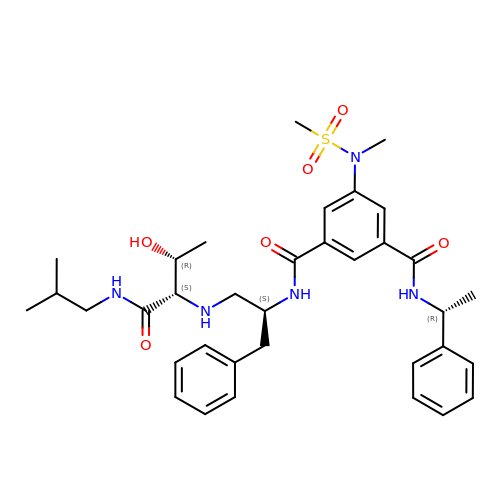N-[(2S)-1-({(2S,3R)-3-hydroxy-1-[(2-methylpropyl)amino]-1-oxobutan-2-yl}amino)-3-phenylpropan-2-yl]-5-[methyl(methylsulfonyl)amino]-N'-[(1R)-1-phenylethyl]benzene-1,3-dicarboxamide | C35 H47 N5 O6 S | UZFAOTIMARRSKT-TYUOOWEOSA-N>[2x]GAMDPMYDISVFIGRFQPFHKGHLHNIIIALQNSKKVIINIGSCFNTPNIKNPFSFEQRKQMIESDLQVAGIDLDTVVIEPLADY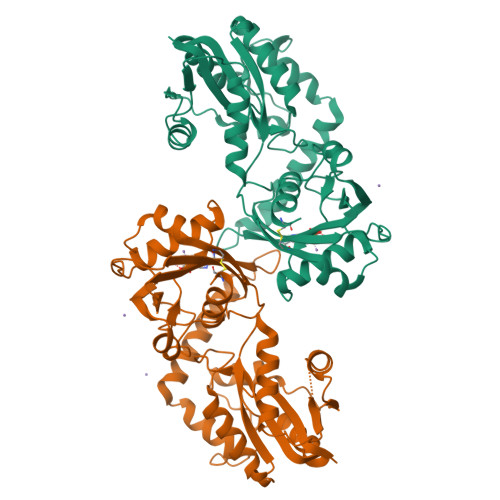FYQEQKWQDELRKNVYKHAKNNNSIAIVGHIKDSSSYYIRSFPEWDYIGVDNYKNFNATEFRQKFYNGIISKQYMCSNDPKLGTYNFLTKFMDTQVYQDLVAENNYVIEYKRLWLKAPFKPNFVTVDALVIVNDHILMVQRKAHPGKDLWALPGGFLECDETIAQAIIRELFEETNINLTHEQLAIAKRCEKVFDYPDRSVRGRTISHVGLFVFDQWPSLPEINAADDAKDVKWISLGSNIKNICDRMLEDHYQIITILLEECGKKL(1S,5S,6R)-10-[S-[3,5-bis(chloranyl)phenyl]-N-methyl-sulfonimidoyl]-5-ethenyl-3-(pyridin-2-ylmethyl)-3,10-diazabicyclo[4.3.1]decan-2-one 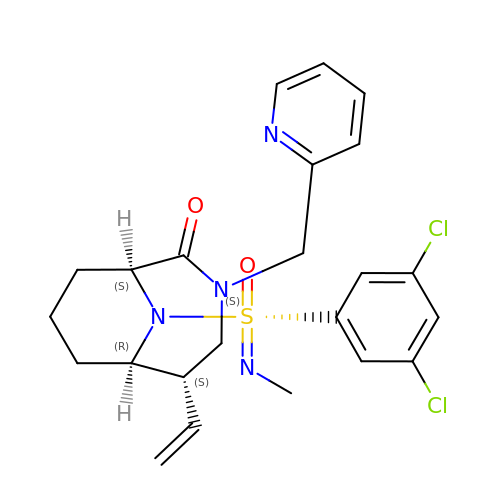| C23 H26 Cl2 N4 O2 S | DQVUTGFTLVPMDO-WVGZOYKRSA-N> MIHAVLIFNKKCQPRLVKFYTPVDLPKQKLLLEQVYELISQRNSDFQSSFLVTPPSLLLSNENNNDEVNNEDIQIIYKNYATLYFTFIVDDQESELAILDLIQTFVESLDRCFTEVNELDLIFNWQTLESVLEEIVQGGMVIETNVNRIVASVDELNKAAESTDSK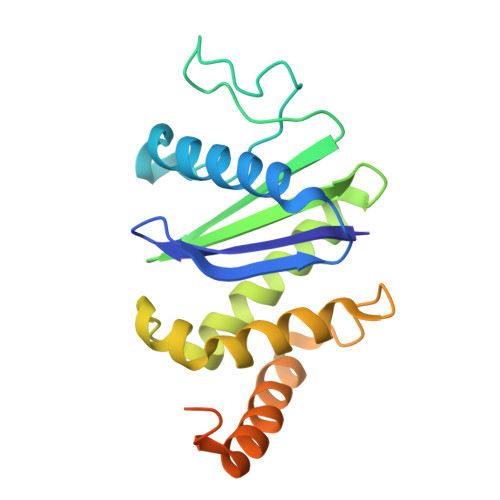IGRLTSTGFGSALQAFAQGGFAQWATGQ> MSEIGTGFPFDP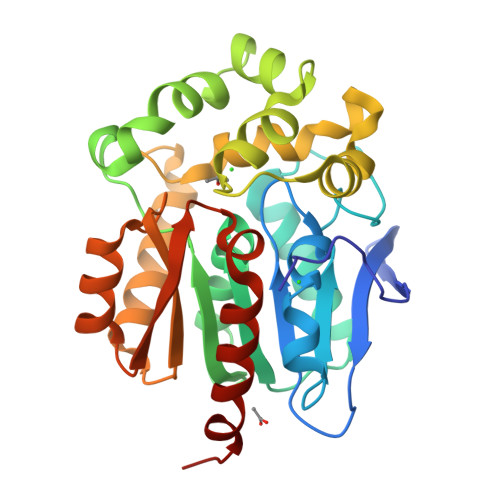HYVEVLGERMHYVDVGPRDGTPVLFLHGNPTSSYLWRNIIPHVAPSHRCIAPDLIGMGKSDKPDLDYFFDDHVRYLDAFIEALGLEEVVLVIHDWGSALGFHWAKRNPERVKGIACMEFIRPFPTWDEWPEFARETFQAFRTADVGRELIIDQNAFIEGALPKYVVRPLTEVEMDHYREPFLKPVDREPLWRFPNELPIAGEPANIVALVEAYMNWLHQSPVPKLLFWGTPGVLIPPAEAARLAESLPNCKTVDIGPGLHYLQEDNPDLIGSEIARWLPALHHHHHH>QGMKTRLEQVLERYLNGREVAVWGVPTRRLLRALKPFKFHTADRVDPQYHYVVAVTDDDL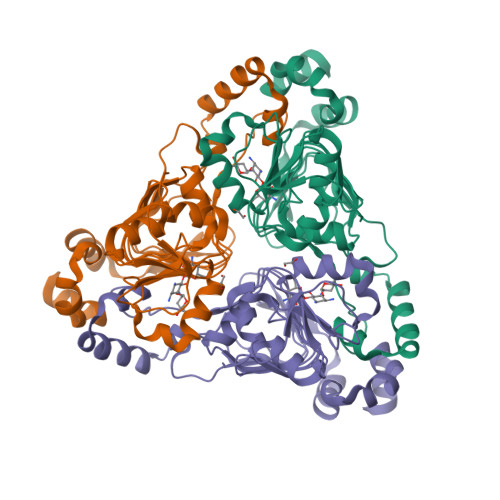TDFLSDEQSKSFQYANDYLTFDDEGGELPFERMCFNVPVGRQTYFGDGVVGACENGYIKSIGQFTSINGTAEIHANAQLNMTFVSDDIQNFFNEESMAVFQEKLRKDPKHPYAYSKEPMTIGSDVYIGAHAFINASTVTSIGDGAIIGSGAVVLENVPPFAVVVGVPARIKRYRFSKEMIETLLRVKWWDWSIEEINENVDALISPELFMKKYGSL[3x]>VSQNQIDDALNGLTTVKVQFDEGIAWVSLNRPDKRNAMSPTLNREMLQVLEALEFDDRCGVVVLTGEGDSFSAGMDLKEYFRETDNAPALIKAQIRRAAGAWQWRKLRFYAKPTIAMVNGWCFGGAFTPLIACDLAVAA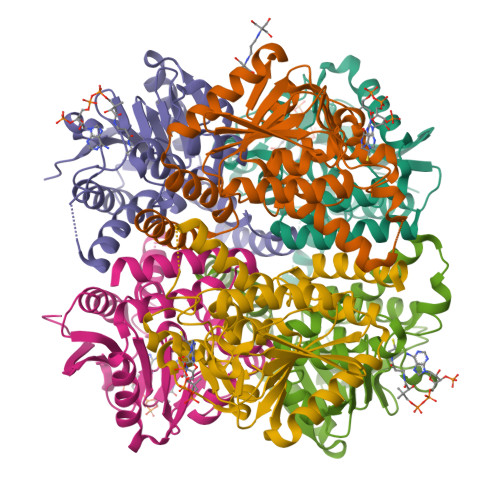DEATFGLSEINWGIIPAGNVTKAVSQVCGERAALYYIMSGEPFGGQKAREIGLVNESVPLAALRERTRELAKTLLGKNPTVLRQAKHALRRVEPMDWDLSEEYLAAKAEQTAAIDPEKGRTKGMKQFLDDKTIRPGLEGYRRGE[6x]> HMPISKKSFLQHVEELCTNNNLKFQEEFSELPKFLQDLSSTDADLPWNRAKNRFPNIKPYNNNRVKLIADASVPGSDYINASYISGYLCPNEFIATQGPLPGTVGDFWRMVWETRAKTLVMLTQCFEKGRIRCH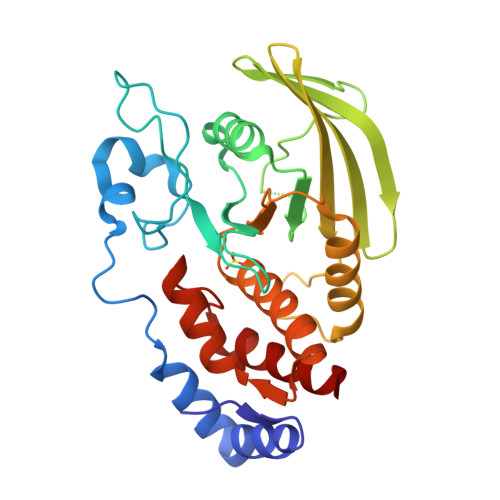QYWPEDNKPVTVFGDIVITKLMEDVQIDWTIRDLKIERHGDCMTVRQCNFTAWPEHGVPENSAPLIHFVKLVRASRAHDTTPMIVHSSAGVGRTGVFIALDHLTQHINDHDFVDIYGLVAELRSERMCMVQNLAQYIFLHQCILDLL> MQREEKQLEASLDALLSQVADLKNSLGSFICKLENEYGRLTWPSVLDSFALLSGQLNTLNKVLKHEKTPLFRNQVIIPLVLSPDRDEDLMRQTEGRVPVFSHEVVPDHLRTKPDPEVEEQEKQLTTDAARIGADAAQKQIQSLNKMCSNLLEKISKEERESESGGLRPNKQTFNPTDTNALVAAVAFGKGLSNWRPSGSSGPGQAGQPGAGTILAGTSGLQQVQMAGA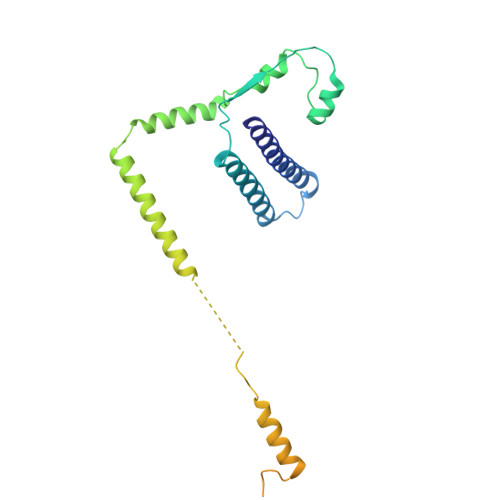PSQQQPMLSGVQMAQAGQPGKMPSGIKTNIKSASMHPYQR> AERGELDLTGAKQNTGVWLVKVPKYLSQQWAKASGRGEVGKLRIAKTQGRTEVSFTLNEDLANIHDIGGKPASVSAPREHPFVLQSVGGQTLTVFTESSSDKL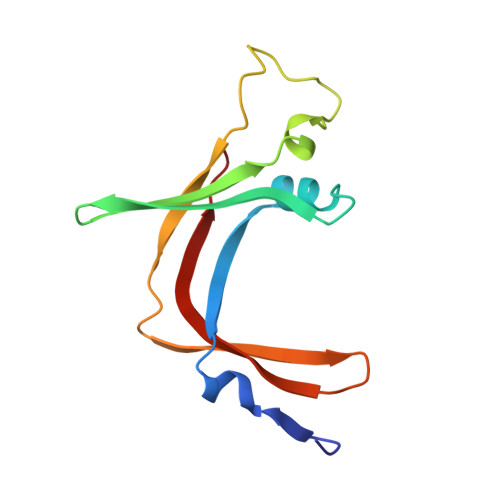SLEGIVVQRAECRPA> MLMRTDPFRDLDRFAQQVLGTSARPAVMPMDAWREGDKFVVEFDLPG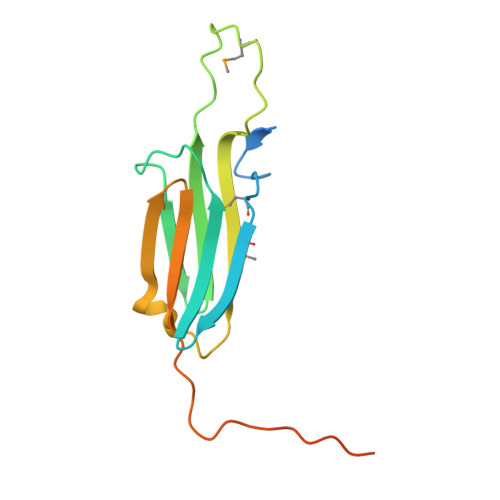IDADSLDIDIERNVVTVRAERPAVDPNREMLASERPRGVFSRQLVLGENLDTARIAASYTEGVLKLQIPVAEKAKPRKISITRGAGDKTISENGAHPEVIEA> GTSTQTKAGSLTIVGTGIESIGQMTLQALSYIEAAAKVFYCVIDPATEAFILTKNKNCVDLYQYYDNGKSRLNTYTQMSELMVREVRKGL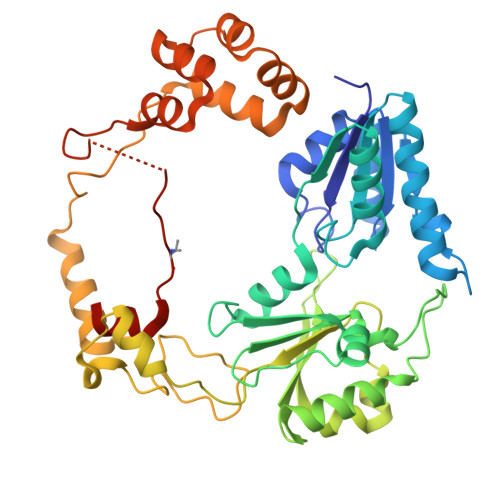DVVGVFYGHPGVFVNPSHRALAIAKSEGYRARMLPGVSAEDCLFADLCIDPSNPGCLTYEASDFLIRDRPVSIHSHLVLFQVGCVGIADFNFTGFDNNKFGVLVDRLEQEYGAEHPVVHYIAAMMPHQDPVTDKYTVAQLREPEIAKRVGGVSTFYIPPKARKASNLDIIRRLELLPAGQVPDKKARIYPANQWEPDVPEVEPYRPSDQAAIAQLADHAPPEQYQPLATSKAMSDVMTKLALDPKALADYKADHRAFAQSVPDLTPQERAALELGDSWAIRCAMKNMPSSLLDAARESGEEASQNGFPWVIVEGVIGVIGSVMSTE>[2x]NVIIGNQKLTINDVARVARNGTLVSLTNNTDILQGIQASCDYINNAVESGEPIFGVTSGFGGMANVAISREQASELQTNLVWFLKTGAGNKLPLADVRAAMLLRANSHMRGASGIRLELIKRMEIFLNAGVTPYVYEFGSIGASGDLVPLSYITGSLIGLDPSFKVDFNGKEMDAPTALRQLNLSPLTLLPKEGLAMMNGTSVMTGIAANCVYDTQILTAIAMGVHALDIQALNGTNQSFHPFIHNSKPHPGQLWAADQMISLLANSQLVRDELDGKHDYRDHELIQDRYSLRCLPQYLGPIVDGISQIAKQIEIE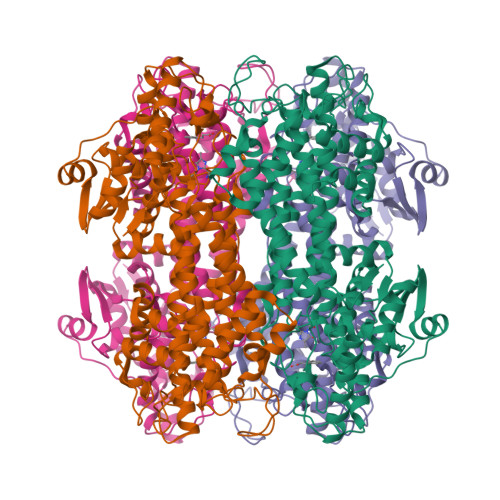INSVTDNPLIDVDNQASYHGGNFLGQYVGMGMDHLRYYIGLLAKHLDVQIALLASPEFSNGLPPSLLGNRERKVNMGLKGLQICGNSIMPLLTFYGNSIADRFPTHAEQFNQNINSQGYTSATLARRSVDIFQNYVAIALMFGVQAVDLRTYKKTGHYDARASLSPATERLYSAVRHVVGQKPTSDRPYIWNDNEQGLDEHIARISADIAAGGVIVQAVQDIL>GENLRPVVINGSNVAMSHGNKEVFSCRGIKLAVDWFLERGHKDITVFVPAWRKEQSRPDALITDQEILRKLEKEKILVFTPSRRVQGRRVVCYDDRFIVKLAFESDGIIVSNDNYRDLANEKPEWKKFIDERLLMYSFVNDKFMPPDDPLGRHGPSLDNFLRKKPIVPEHKKQPCPYG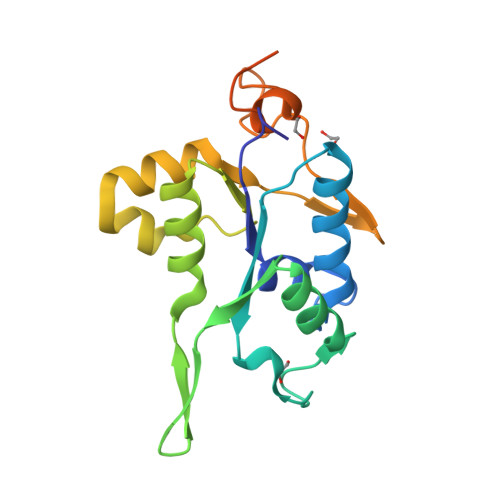KKCTYGHKCKYYHP[2x]>SSSESLSIIDVASDQNLFQTFIKEWRCKKRFSISLACEKIRSLTSSKTATIGSRFKQASSPQEIPIRDDGFPIKGCDDTLVVGLAVCWGGRDAYYFSLQKEQKHSEISASLVPPSLDPSLTLKDRMWYLQSCLRKESDKECSVVIYDFIQSYKILLLSCGISLEQSYEDPKVACWLLDPDSQEPTLHSIVTSFLPHELPLLEGMETSQGIQSLGLNAGSEHSGRYRASVESILIFNSMNQLNSLLQKENLQDVFRKVEMPSQYCLALLELNGIGFSTAECE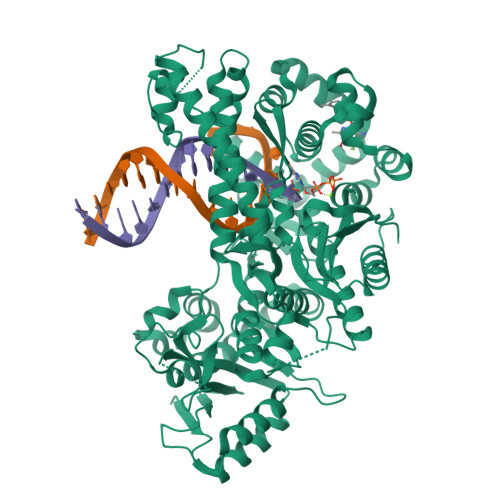SQKHIMQAKLDAIETQAYQLAGHSFSFTSSDDIAEVLFLELKLPPNREMKNQGSKKTLGSTRRGIDNGRKLRLGRQFSTSKDVLNKLKALHPLPGLILEWRRITNAITKVVFPLQREKCLNPFLGMERIYPVSQSHTATGRITFTEPNIQNVPRDFEIKMGGMPFSISMRHAFVPFPGGSILAADYSQLELRILAHLSHDRRLIQVLNTGADVFRSIAAEWKMIEPESVGDDLRQQAKQICYGIIYGMGAKSLGEQMGIKENDAACYIDSFKSRYTGINQFMTETVKNCKRDGFVQTILGRRRYLPGIKDNNPYRKAHAERQAINTIVQGSAADIVKIATVNIQKQLETFHSTFKSHGHREGMLQSDQTGLSRKRKLQGMFCPIRGGFFILQLHDELLYEVAEEDVVQVAQIVKNEMESAVKLSVKLKVKVKIGASWGELKDFDV[6x]>MQNQLYIDGRFVDAVAGGTIDVVSPHDGSLITRIAAAEAADVDLAVAAAKRAFPAWSALGAAERGRLLLKLADRIEECSEELAQLESLNTGHPIRDSRGLDVPRTAACFRYFGGMADKIEGSVIPVDAGFLNYVQRKPIGVVAQIVPWNFPLMFTSWKMGPALAAGNTIVIKPSEITPLSTLRIVELMTEVGFPKGVVNVVPGYGHTAGQALAEHLDVGKIAFTGSTATGRRIVEASKSNLKRIQLELGGKGANIVFEDANIEAAVNGAAWAIFHNQGQACIAGSRLILHKDIADQFLERFIALAKSIRLGDPMDPETEMGPLTSALRRDRVLSYIDIAIEQGGKVLAGGKAPDDKALANGFYVEPTVVEAKPQDRVCQEEVFGPFVTVVRFSSDEEALAIANNTEYGLGSGLWTQNLARAHKMAHAIHAGMCWINCYKRVSPGSPFGGVGQSGYGREMGFEAIHDYTEARSVWVNVDAKIAPHFKRLGHHHH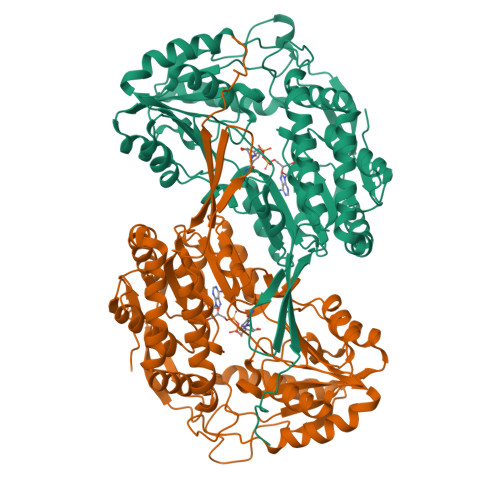HH[8x]> MLLGSSEESQAFQRQLTALIGYDVTDVSNVHDDELEFTRRGLVTPRMAEVASRDPKLYAMHPWVTSKPLPEYLWKKIANNCIFIVIHRSTTSQTIKVSPDDTPGAILQSFFTKMAKKKSLMDIPESQSEQDFVLRVCGRDEYLVGETPIKNFQWVRHCLKNGEEIHVVLDTPPDPALDEVRKEEWPLVDDCTGVTGYHEQLTI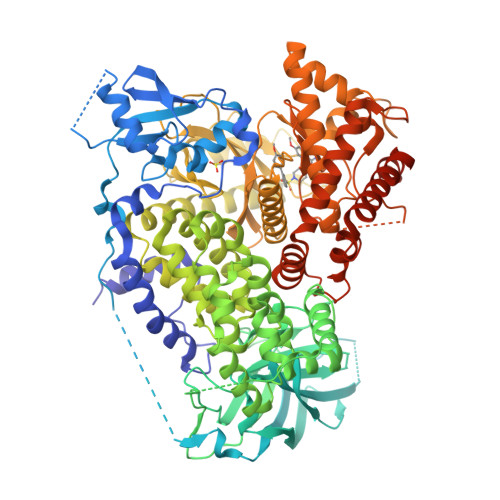HGKDHESVFTVSLWDCDRKFRVKIRGIDIPVLPRNTDLTVFVEANIQHGQQVLCQRRTSPKPFTEEVLWNVWLEFSIKIKDLPKGALLNLQIYCGKAPALSSKASAESPSSESKGKVQLLYYVNLLLIDHRFLLRRGEYVLHMWQISGKGEDQGSFNADKLTSATNPDKENSMSISILLDNYCHPIALPKHQPTPDPEGDRVRAEMPNQLRKQLEAIIATDPLNPLTAEDKELLWHFRYESLKHPKAYPKLFSSVKWGQQEIVAKTYQLLARREVWDQSALDVGLTMQLLDCNFSDENVRAIAVQKLESLEDDDVLHYLLQLVQAVKFEPYHDSALARFLLKRGLRNKRIGHFLFWFLRSEIAQSRHYQQRFAVILEAYLRGCGTAMLHDFTQQVQVIEMLQKVTLDIKSLSAEKYDVSSQVISQLKQKLENLQNSQLPESFRVPYDPGLKAGALAIEKCKVMASKKKPLWLEFKCADPTALSNETIGIIFKHGDDLRQDMLILQILRIMESIWETESLDLCLLPYGCISTGDKIGMIEIVKDATTIAKIQQSTVGNTGAFKDEVLNHWLKEKSPTEEKFQAAVERFVYSCAGYCVATFVLGIGDRHNDNIMITETGNLFHIDFGHILGNYKSFLGINKERVPFVLTPDFLFVMGTSGKKTSPHFQKFQDICVKAYLALRHHTNLLIILFSMMLMTGMPELTSKEDIEYIRDALTVGKNEEDAKKYFLDQIEVCRDKGWTVQFNWFLHLVLGIKQGEKHSAEFGLVPRGSGHHHHHH> IRQNYSTEVEAAVNRLVNLYLRASYTYLSLGFYFDRDDVALEGVCHFFRELAEEKREGAERLLKMQNQRGGRALFQDLQKPSQDEWGTTPDAMKAAIVLEKSLNQALLDLHALGSAQADPHLCDFLESHFLDEE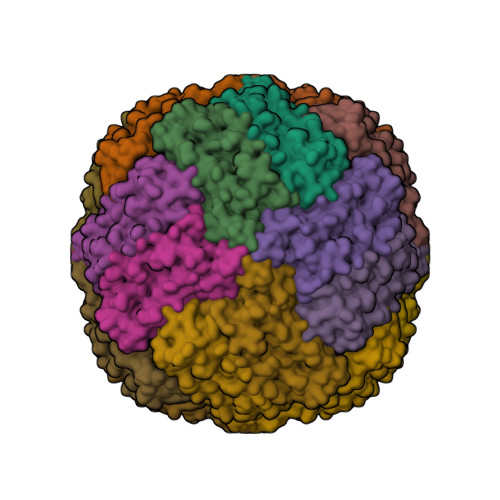VKLIKKMGDHLTNIQRLVGSQAGLGEYLFERLTLKHD>[2x]AATYAQTLQNIPETNVTTLDNGLRVASEESSQPTCTVGVWIGAGSRYENEKNNGAGYFVEHLAFKGTKKRPCAAFEKEVESMGAHFNGYTSREQTAFYIKALSKDMPKVVELLADVVQNCALEESQIEKERGVILQELKEMDNDMTNVTFDYLHATAFQGTALARTVEGTTENIKHLTRADLASYIDTHFKAPRMVLAAAGGISHKELVDAARQHFSGVSFTYKEDAVPILPRCRFTGSEIRARDDALPVAHVALAVEGPGWADPDNVVLHVANAIIGRYDRTFGGGKHLSSRLAALAVEHKLCHSFQTFNTSYSDTGLFGFHFVADPLSIDDMMFCAQGEWMRLCTSTTESEVKRAKNHLRSAMVAQLDGTTPVCETIGSHLLNYGRRISLEEWDSRISAVDARMVRDVCSKYIYDKCPALAAVGPIEQLLDYNRIRSGMYWIRF;>[2x]SLKVAPKVAVSAAAERVKLCPGAEDLEITKLPNGLIIASLENFSPASRIGVFIKAGSRYETTANLGTAHLLRLASPLTTKGASSFRITRGIEAVGGSLSVYSTREKMTYCVECLRDHVDTVMEYLLNVTTAPEFRPWEVTDLQPQLKVDKAVAFQSPQVGVLENLHAAAYKTALANPLYCPDYRIGKITSEQLHHFVQNNFTSARMALVGIGVKHSDLKQVAEQFLNIRSGAGTSSAKATYWGGEIREQNGHSLVHAAVVTEGAAVGSAEANAFSVLQHVLGAGPLIKRGSSVTSKLYQGVAKATTQPFDASAFNVNYSDSGLFGFYTISQAAHAGEVIRAAMNQLKAAAQGGVTEEDVTKAKNQLKATYLMSVETAQGLLNEIGSEALLSGTHTAPSVVAQKIDSVTSADVVNAAKKFVSGKKSMAASGDLGSTPFLDEL;>[2x]MAPNIRKSHPLLKMINNSLIDLPAPSNISAWWNFGSLLAVCLMTQILTGLLLAMHYTADTSLAFSSVAHTCRNVQYGWLIRNLHANGASFFFICIFLHIGRGLYYGSYLYKETWNTGVILLLTLMATAFVGYVLPWGQMSFWGATVITNLFSAIPYIGHTLVEWAWGGFSVDNPTLTRFFALHFLLPFAIAGITIIHLTFLHESGSNNPLGISSDSDKIPFHPYYSFKDILGLTLMLTPFLTLALFSPNLLGDPENFTPANPLVTPPHIKPEWYFLFAYAILRSIPNKLGGVLALAASVLILFLIPFLHKSKQRTMTFRPLSQTLFWLLVANLLILTWIGSQPVEHPFIIIGQMASLSYFTILLILFPTIGTLENKMLNY;>[2x]GELELHPPAFPWSHGGPLSALDHSSVRRGFQVYKQVCSACHSMDYVAFRNLIGVTHTEAEAKALAEEVEVQDGPDENGELFMRPGKISDYFPKPYPNPEAARAANNGALPPDLSYIVNARHGGEDYVFSLLTGYCDPPAGVVVREGLHYNPYFPGQAIGMAPPIYNEILEYDDGTPATMSQIAKDVCTFLRWAAEPEHDQRKRMGLKMLLISALLTSLLYYMKRHKWSVLKSRKMAYRPPK;>[2x]VHNDVTVPDFSAYRREDVMDATTSSQTSSEDRKGFSYLVTATACVATAYAAKNVVTQFISSLSAS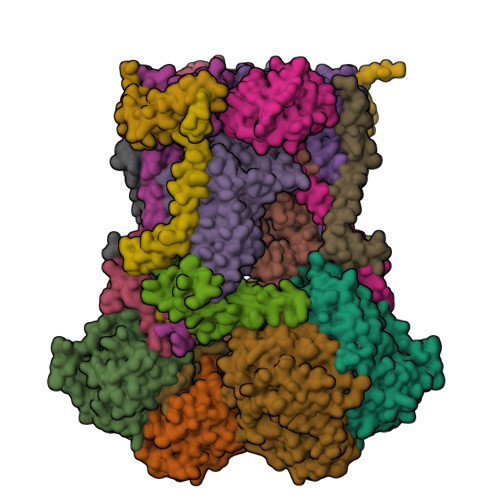ADVLALSKIEIKLSDIPEGKNVAFKWRGKPLFVRHRTQAEINQEAEVDVSKLRDPQHDLDRVKKPEWVILVGVCTHLGCVPIANSGDFGGYYCPCHGSHYDASGRIRKGPAPYNLEVPTYQFVGDDLVVVG;>[2x]AARATVAGGGRLMDRIRKWYYNAAGFNKYGLMRDDTLYEDDDVKEALKRLPEDLYNERMFRIKRALDLSLKHRILPKEQWVKYEEDKPYLEPYLKEVIRERLEREAWNKK;>[2x]GIHFGNLARVRHIITYSLSPFEQRAIPNIFSDALPNVWRRFSSQVFKVAPPFLGAYLLYSWGTQEFERLKRKNPADYENDQ;>LRGSGEEEEEELVDPLTTIREHCEQTEKCVKARERLELCDARVSSRSHTEEQCTEELFDFLHARDHCVAHKLFNKLK[2x];>[2x]ALLRQAYSALFRRTSTFALTVVLGAVLFERAFDQGADAIFEHLNEGKLWKHIKHKYEASEE> PREEKAQAALFKGQEYFEQDAYEQALNGDSIGYVGFLKVADEYSGTKAANLAKAYAGICYAQLGKYDEAVKMLDGFNGGDQMVAPAILGATGNCYAQLGQLDKAASTLLSAADKADNNSLSPIFLMQAG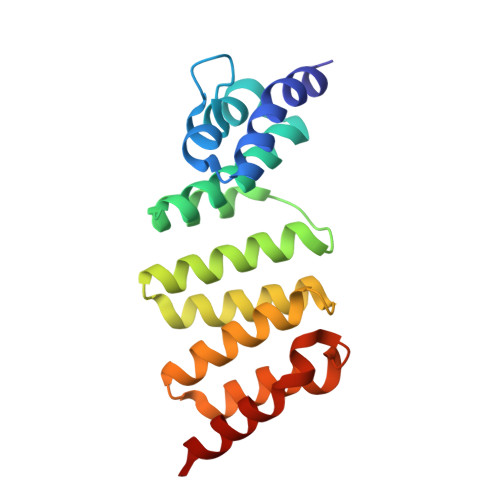EILVKQGKYDDAVNAYTKIKDKYFQSYQAMDIDKYIEQAKLMKK1-(beta-D-glucopyranosyl)-5-(trifluoromethyl)pyrimidine-2,4(1H,3H)-dione 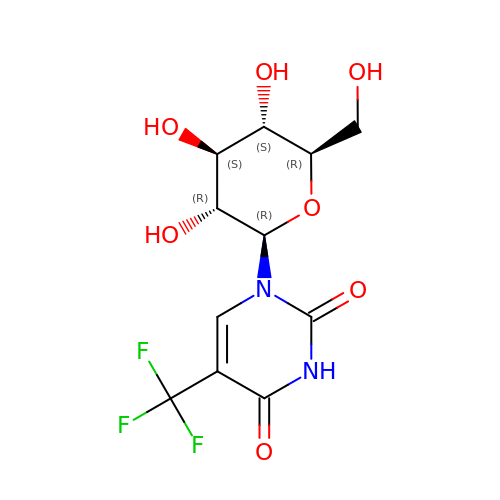| C11 H13 F3 N2 O7 | NADUQTKHANBUDE-XSEHCYKFSA-N> SPTRLTYISDIIEISPYLRRLV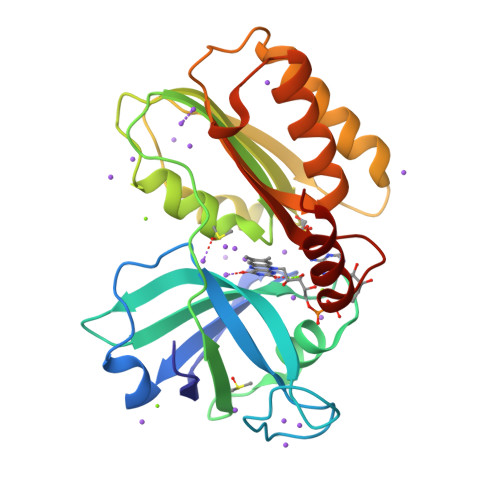LSGEQLANFPADQQGAYVKVLIPQPGETTVNMTLTGPNAAIKRSYTIREFDPVRGQLSLDFVINKHTGPATDWAKLANVGDTVAIAGPGPLKMNRFDFNDYLLFGDSTSINAVDALIKRLPATAKGHIIMLVNSHQEQALLSQHPLLKTHWLVLNDSITAEQQIDWLLDKLELFGDLPAVTQVFVGLEATQVRVIKQYLLEQQQLPLSSISATGYWKRNTDADTFGKQKQMQPL>APAAVDWRARGAVTAVKDQGQCGSCWAFSAIGNVECQWFLAGHPLTNLSEQMLVSCDKTDSGCSGGLMNNAFEWIVQENNGAVYTEDSYPYASGEGISPPCTTSGHTVGATITGHVELPQDEAQIAAWLAVNGPVAVAVDASSWMTYTGGVMTSCVSEQLDHGVLLVGYNDSAAVPYWIIKNSWTTQWGEEGYIRIAKGSNQCLVK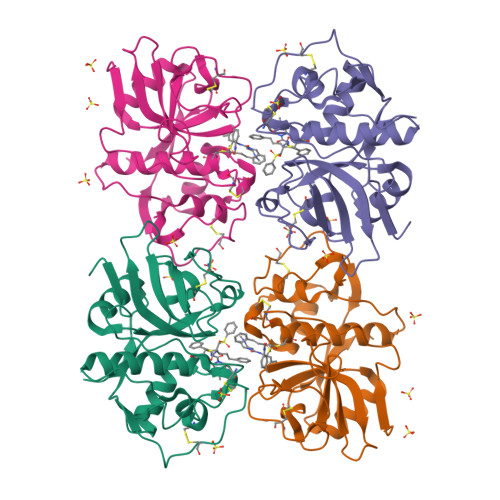EEASSAVVG[2x]>[4x]GAMGSPSSQKALLLELKGLQEEPVEGFRVTLVDEGDLYNWEVAIFGPPN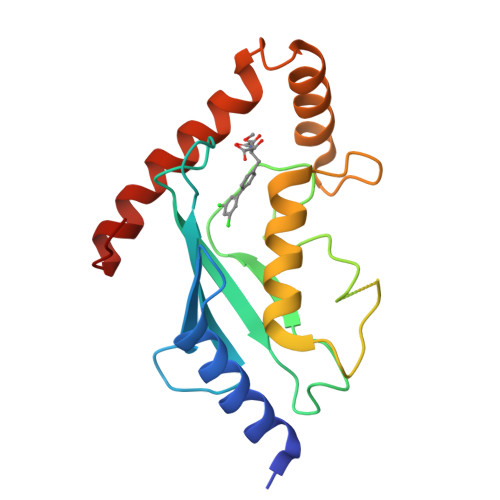TYYEGGYFKARLKFPIDYPYSPPAFRFLTKMWHPNIYETGDVCISILHPPVDDPQSGELPSERWNPTQNVRTILLSVISLLNEPNTFSPANVDASVMYRKWKESKGKDREYTDIIRKQVLGTKVDAERDGVKVP>[2x]MVATPVKQKYDIKDISLAPQGRQEIEWAAREMPVLKQIRERFAQEKPFAGIRLVACCHVTTETANLAIALHAGGADSLLIASNPLSTQDDVAACLVADYGIPVYAIKGEDNETYHRHVQIALDHRPNIIIDDGSDVVATLVQERQHQLSD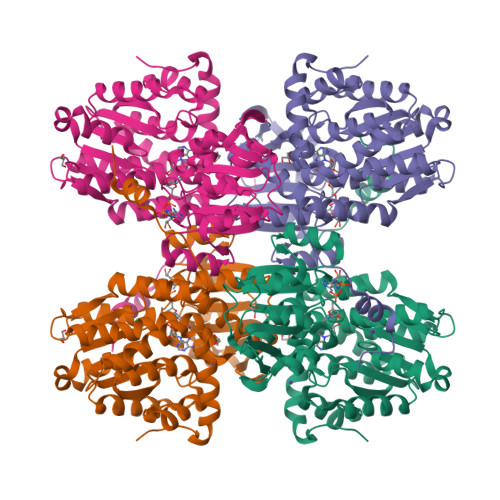IIGTTEETTTGIVRLRAMFNDGVLTFPAMNVNDADTKHFYDNRYGTGQSTLDGIIRATNILLAGKTIVVAGYGWCGKGVAMRAKGMGADVIVTEISPVPAIEAAMDGFRVMPMAEAAHQGDIFITVTGNKHVIRPEHFAVMKDGAIVCNSGHFDIEIDLKSLKEQAKEVKEVRNFTEQYILPNGKSIIVIGEGRLVNLAAAEGHPSAVMDMSFANQALACEHLVKNKGQLEPGMHSIPVEVDQEIARLKLQAMGIAIDSLTPEQVEYINSWASGT>GPVGYGAATTGGGNKVPVNVATFEAMQSAIDSYSGSGGLVLNYTGKFDFGTIKDVCAQWKLPAKTVQIKNKSDVTIKGANGSAANFGIRVVGNAHNVIIQNMTIGLLQGGEDADSISLEGNSSGEPSKIWVDHNTVFASLTKCSGAGDASFDGGIDMKKGVHHVTVSYNYVYNYQKVALNGYSDSDTKNSAARTTYHHNRFENVESRVPLQRFGLSHIYNNYFNNVTTSGINVRMGGIAKIESNYFENIKNPVTSRDSSEI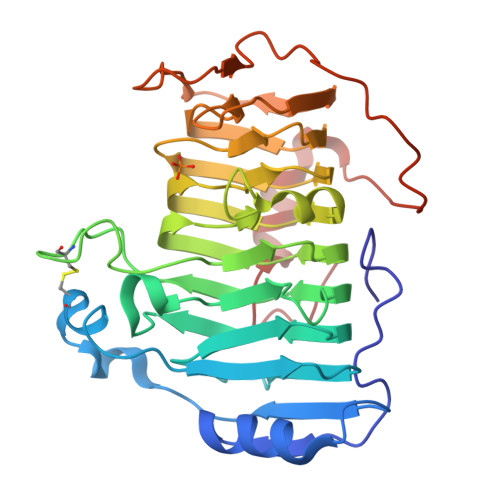GYWDLINNYVGSGITWGTPDGSKPYANATNWISTKVFPESLGYIYTVTPAAQVKAKVIATAGAGKNLAE[2x]>[2x]GMSENSSVRHGLTSAQHCVWLAQQLDPRGAHYRTGSCLEIDGPLDHAVLSRALRLTVAGTETLCSRFLTDEEGRPYRAYCPPAPEGSAAVEDPDGVPYTPVLLRHIDLSGHE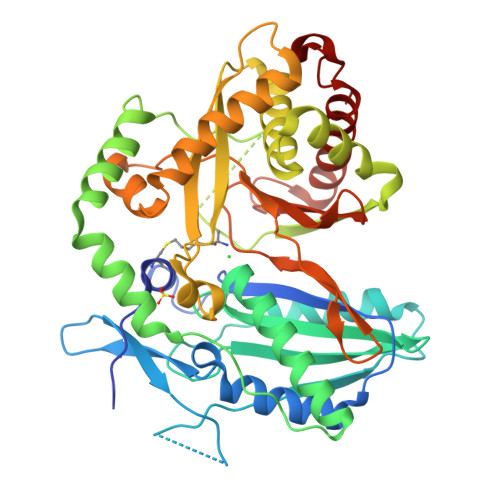DPEGEAQRWMDRDRATPLPLDRPGLSSHALFTLGGGRHLYYLGVHHIVIDGTSMALFYERLAEVYRALRDGRAVPAAAFGDTDRMVAGEEAYRASARYERDRAYWTGLFTDRPEPVSLTGRGGGRALAPTVRSLGLPPERTEVLGRAAEATGAHWARVVIAGVAAFLHRTTGARDVVVSVPVTGRYGANARITPGMVSNRLPLRLAVRPGESFARVVETVSEAMSGLLAHSRFRGEDLDRELGGAGVSGPTVNVMPYIRPVDFGGPVGLMRSISSGPTTDLNIVLTGTPESGLRVDFEGNPQVYGGQDLTVLQERFVRFLAELAADPAATVDEVALLT> MAPLRK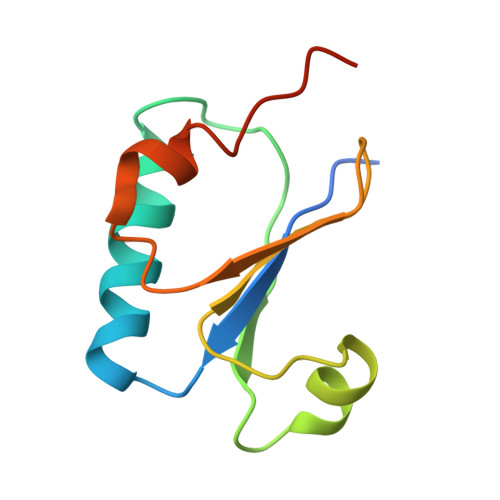TAVLKLYVAGNTPNSVRALKTLNNILEKEFKGVYALKVIDVLKNPQLAEEDKILATPTLAKVLPPPVRRIIGDLSNREKVLAGLDLLAEEIGD> GPVSVANHLGEDAGHLALRRDVYSGLQKTPKSLPPKWFYDTVGSELFDQITRLPEYYPTRAEAEILRARSAEVASACRADTLVELGSGTSEKTRMLLDALRHRGSLRRFVPFDVDASVLSATATAIQREYSGVEINAVCGDFEEHLTEIPRGGRRLFVFLGSTIGNLTPGPRAQFLTALAGVMRPGDSLLLGTDLVKDAARLVRAYDDPGGVTAQFNRNVLAVINRELEADFDVDAFQHVARWNSAEERIEMWLRADGRQRVRVGALDLTVDFDAGEEM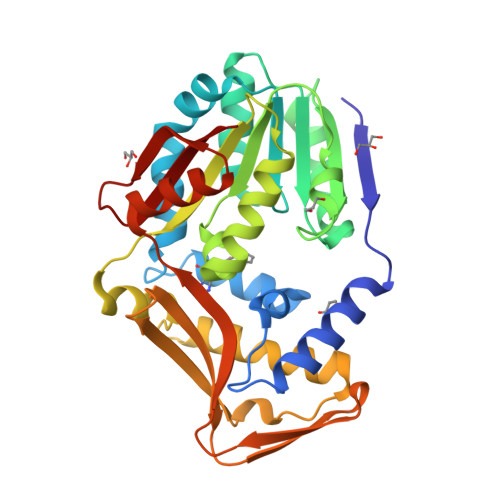LTEVSCKFRPQAVGAELAAAGLHRIRWWTDEAGDFGLSLAAK(3R)-3-{3-[(2H-1,3-benzodioxol-5-yl)methyl]-1,2,4-oxadiazol-5-yl}-4-cyclopentyl-N-hydroxybutanamide 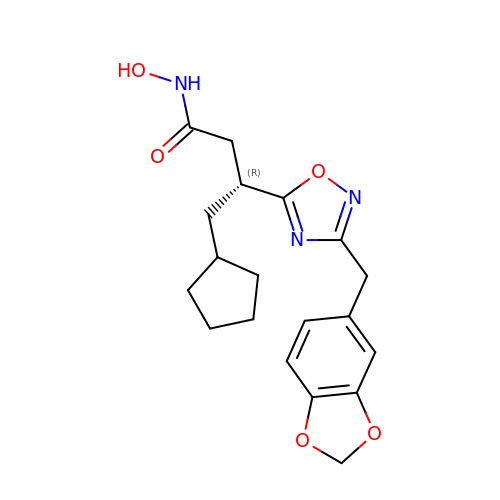| C19 H23 N3 O5 | XOZSWEYBEQSKBV-CQSZACIVSA-N> MKIGVFVPIGNNGWLISTHAPQYMPTFELNKAIVQKAEHYHFDFALSMIKLRGFGGKTEFWDHNLESFTLMAGLAAVTSRIQIYATAATLTLPPAIVARMAATIDSISGGRFGVNLVTGWQKPEYEQMGIWPGDDYFSRRYDYLTEYVQVLRDLWGTGKSDFKGDFFTMNDCRVSPQPSVPMKVICAGQSDA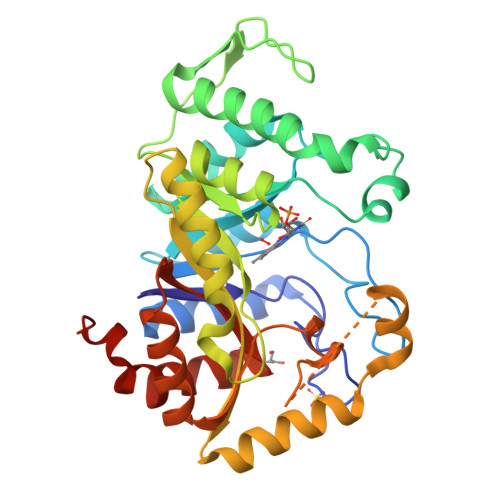GMAFSARYADFNFCFGKGVNTPTAFAPTAARMKQAAEQTGRDVGSYVLFMVIADETDDAARAKWEHYKAGADEEALSWLTEQSQKDTRSGTDTNVRQMADPTSAVNINMGTLVGSYASVARMLDEVASVPGAEGVLLTFDDFLSGIETFGERIQPLMQCRAHLPALTQEVA3-[[3-(trifluoromethyl)phenyl]methyl]-2~{H}-1$l^{6},2,4-benzothiadiazine 1,1-dioxide | C15 H11 F3 N2 O2 S | 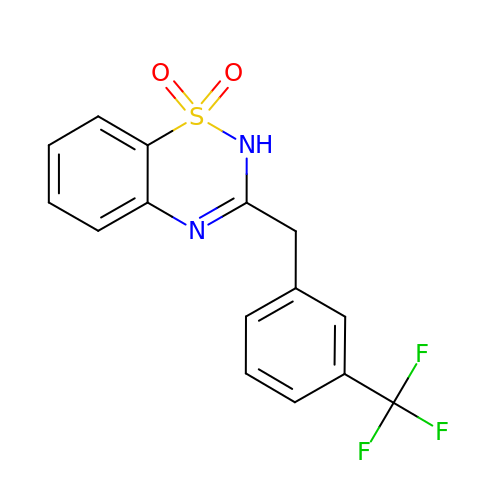IXHISIYNGIIOEL-UHFFFAOYSA-N> SMGAEPGRPARLDQLLDMPAAGLAVQLRHAWNPEDRSLNVFVKDDDRLTFHRHPVAQSTDGIRGKVGHARGLHAWQINWPARQRGTHAVVGVATARAPLHSVGYTALVGSDAESWGWDLGRSRLYHDGKNQPGVAYPAFLGPDEAFALPDSLLVVLDMDEGTLSFIVDGQYLGVAFRGLKGKKLYPVVSAVWGHCEVTMRYINGLDPE

The SPRY domain- and SOCS box-containing proteins, SPSB1 to SPSB4 (also known as SSB-1 to -4), contain a protein interaction domain known as the SPRY domain, which was first identified as a sequence repeat in the dual-specificity kinase splA and ryanodine receptors, together with a C-terminal SOCS box motif. The presence of the SOCS box motif suggests that the SPSB proteins may function as part of an E3 ubiquitin ligase, with the SPRY domain determining the substrate(s) for ubiquitination, and this has been confirmed recently for SPSB2 (Z.K., R.S.L., R.S.N., and S.E.N., personal communication). All three hSPSB proteins share the same conserved SPRY domain fold with two short N-terminal helices packed against a bent β-sandwich, comprising two 7-stranded β-sheets. The structures show remarkable conservation of the SPRY domain fold and absolute sequence conservation for positions in contact with the (E/D)(L/I)NNN motif.

The apo-structures of mSPSB2 and hSPSB4 show some additional differences in loop conformation. The most significant change affects loop B, where hSPSB4 Pro79 and Val80 are displaced relative to the corresponding residues in mSPSB2. However, the orientation of the adjacent hSPSB4 Arg77 residue, which would bind the third Asn (hPar-4 Asn72), is essentially unchanged because of its largely buried position in the β3 strand. Loops C (e.g., hSPSB4 Thr111) and E (e.g., hSPSB4 Trp217) are also somewhat displaced relative to mSPSB2, although their overall conformations are similar. Again, a significant rearrangement of the Trp side chain would be required to accommodate the peptide ligand.> HNHNHNHNHNHNGGENLYFQGASLTEIEHLVQSVCKSYRETCQLRLEDLLRQRSNIFSREEVTGYQRKSMWEMWERCAHHLTEAIQYVVEFAKRLSGFMELCQNDQIVLLKAGAMEVVLVRMCRAYNADNRTVFFEGKYGGMELFRALGCSELISSIFDFSHSLSALHFSEDEIALYTALVLINAHRPGLQEKRKVEQLQYNLELAFHHHLCKTHRQSILAKLPP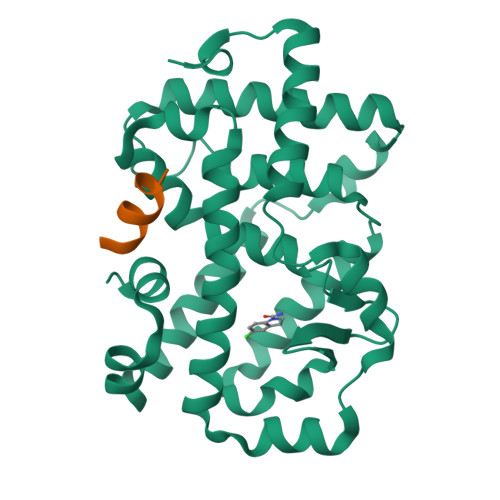KGKLRSLCSQHVERLQIFQHLHPIVVQAAFPPLYKELFSGG;> KILHRLLQDS>MISNDHLKRLASTSAVMSCTLGKATCLGMDKICSPLADNDVTQRKTQIICTIGPSCNNVESLIGLIDKGMSVARLNFSHGDHESHFKTLQNIREAAKARPHSTVGIMLDTKGPEIRTGMLEGGKPIELKAGQTLKITTDYSMLGNSECISCSYSLLPKSVQIGSTVLIADGSLSTQVLEIGDDFIVCKVLNSVTIGERKNMNLPGCKVHLPIIGDKDRHDIVDFALKYNLDFIALSFVQNGADVQLCRQIISENTQYSNGIPSSIKIISKIENLEGVINFDSICSESDGIMVARGDLGMEIPPEKIFVAQKCMISKCNVAGKPVVTATQMLESMIKSNRPTRAEMTDVANAVLDGSDCVMLSGETANGAFPFDAVNVMSRVCAQAETCIDYPVLYHAIHSSVPKPVAVPEAIACSAVESAHDVNAKLIITITETGNTARLISKYRPSQTIIACTAKPEVARGLKIARGVKTYVLNSIHHSEVVISNALALAKEESLIESGDFAIAVHGVKESCPGSCNLMKIVRCP[2x]

PyK catalyzes the last step of glycolysis, in which the phosphoryl group of phosphoenolpyruvate (PEP) is transferred to ADP to form pyruvate and ATP, and serves as a major regulator of glycolysis. Notably, C. parvum PyK (CpPyK) is exceptional, as it showed no allosteric property. However, the majority of PyKs are tetrameric, and CpPyK also displays a tetrameric assembly in the crystal structure. Each CpPyK molecule consists of four domains: N (residues 23–32), A (42–112 and 212–389), B (113–211) and C (390–526).

The asymmetric unit in the crystal structure contains two monomers (A & B) of CpPyK related by non-crystallographic two-fold symmetry. A new feature of the CpPyK structure is that the two monomers in the asymmetric unit are linked by two right-handed disulfide bonds between Cys26 of one monomer and Cys312 of the other. The final model also contains two sulfate ions, SULF1 and SULF2 (corresponding to SO4 527 and SO4 528 in the deposited coordinates), and two glycerol molecules, GOL1 and GOL2 (GOL530 and GOL 531 in the deposited coordinates), associated with each chain. Instead, there is a glycerol molecule (GOL1) located in the active site of CpPyK at nearly the same position occupied by the ATP γ-phosphate. The GOL1 molecule at the ATP binding site in the CpPyK crystal structure, therefore, has a similar effect as the sulfate ion in the active site. Each monomer in the asymmetric unit of CpPyK binds two sulfate ions at equivalent positions, one in the C-domain and the other at the interface of the A and C domains. The sulfate ion in the C-domain (SULF1) occupies a position corresponding to the 6-phosphate of the effector molecule in different PyKs (location E in Fig 4A). In spite of the presence of the sulfate ion, the loop between the two C-terminal β strands in the molecule (residues 508–517) is disordered as seen in other PyK structures without any effector molecule. The second sulfate ion (SULF2) occupies a small pocket at the interface of the A and C domains and is hydrogen-bonded to two NZ atoms (Lys464 and Lys470), the hydroxyl oxygen of Thr471 (all in domain C), and the peptide N atom of Thr103, which belongs to domain A.>[4x]GSDEDTYY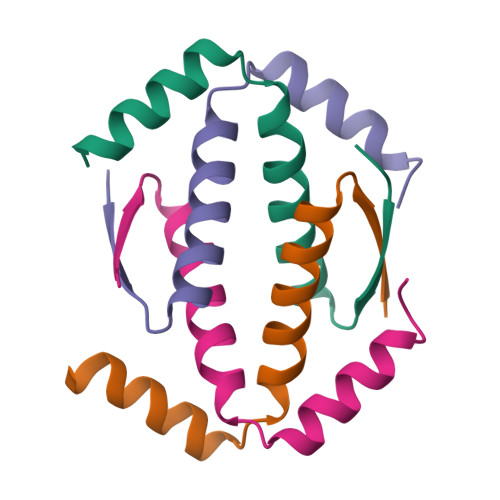LQVRGRENFEILMKLKESLELMELVPQPLVDSYRQQQQLLQRP> MSETQSQTMTRPQDLSLSDINSTVEVPEGHSFWKTLLAYSGPGALVAVGYMDPGNWSTSITGGQNFQYLLLSIIVISSLLAMLLQNMAAKLGIVCQLDLAQAIRARTSRRLGFIFWILTELAIMATDIAAVIGAAIALYLLFKIPIFLAVVITVLDVFLLLLLNRIGFRKIEALVVCLIFVILFVFLYQIILSQPAWHQVAKGLIPSWASVQTSPKIGGQTPLSASLGIIGATIMPHNLFLHSAISQSRKIDRTDSSKVAEAVRFSNWDSNIQLSLAMVVNALLLIMGVAVFKSGAVQDPSFFGLYQALSNPDMVSNPVLAEAARSGVLSTLFAVALLASGQNSTITGTITGQVIMEGFIHLR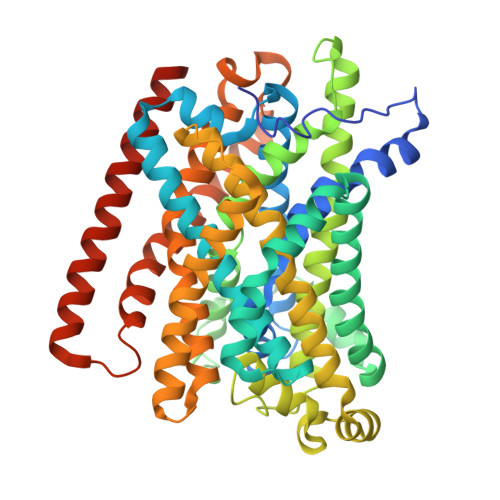LPLWLRRLVTRLIAIIPVVVCVAITSHQGSLDEHQALNNLMNNSQVFLALALPFSIVPLLMLTDSAAQMGNQFKNTRWVKVMGWLTVIILTLLNLISISSQIAGFFGDNPSSQDLLLSQVISIGIILAMIGLLIWTIIDIRRFTHPKQKALEVLFQ>STAGKVIKCKAAVLWEVKKPFSIEDVEVAPPKAYEVRIKMVAVGICRTDDHVVSGNLVTPLPVILGHEAAGIVESVGEGVTTVKPGDKVIPLFTPQCGKCRVCKNPESNYCLKNDLGNPRGTLQDGTRRFTCRGKPIHHFLGTSTFSQYTVVDENAVAKIDAASPLEKVCLIGCGFSTGYGSAVNVAKVTPGSTCAVFGLGGVGLSAVMGCKAAGAARIIAVDINKDKFAKAKELGATECINPQDYKKPIQEVLKEMTDGGVDFSFEVIGRLDT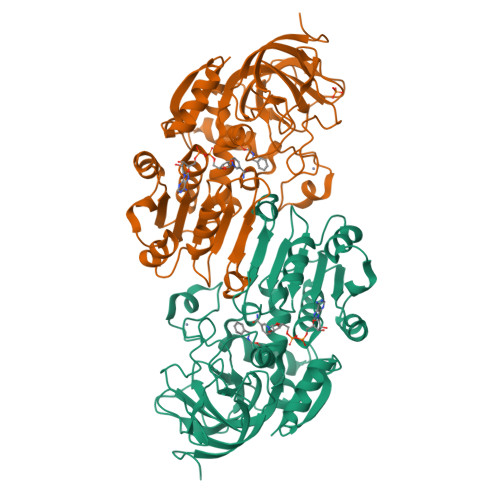MMASLLCCHEACGTSVIVGVPPASQNLSINPMLLLTGRTWKGAVYGGFKSKEGIPKLVADFMAKKFSLDALITHVLPFEKINEGFDLLHSGKSIRTVLTF[2x]>[2x]MEKERETLQAWKERVGQELDRVMAFWLEHSHDREHGGFFTCLGRDGRVYDDLKYVWLQGRQVWMYCRLYRKLERFHRPELLDAAKAGGEFLLRHARVAPPEKKCAFVLTRDGRPVKVQRSIFSECFYTMAMNELWRVT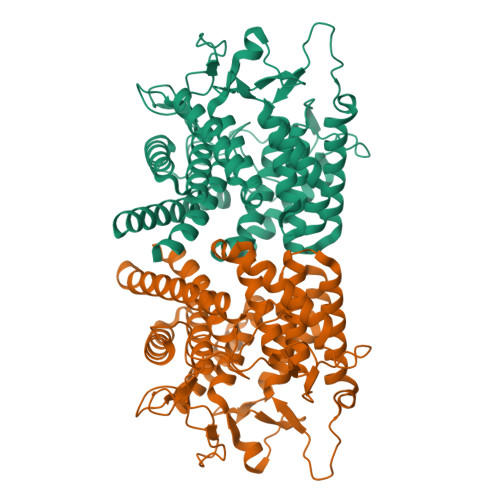AEARYQSEAVDMMDQIVHWVREDPSGLGRPQLPGAVASESMAVPMMLLCLVEQLGEEDEELAGRYAQLGHWCARRILQHVQRDGQAVLENVSEDGEELSGCLGRHQNPGHALEAGWFLLRHSSRSGDAKLRAHVIDTFLLLPFRSGWDADHGGLFYFQDADGLCPTQLEWAMKLWWPHSEAMIAFLMGYSESGDPALLRLFYQVAEYTFRQFRDPEYGEWFGYLNREGKVALTIKGGPFKGCFHVPRCLAMCEEMLSALLSRLA> MSVQAEIGILDHVDGSSEF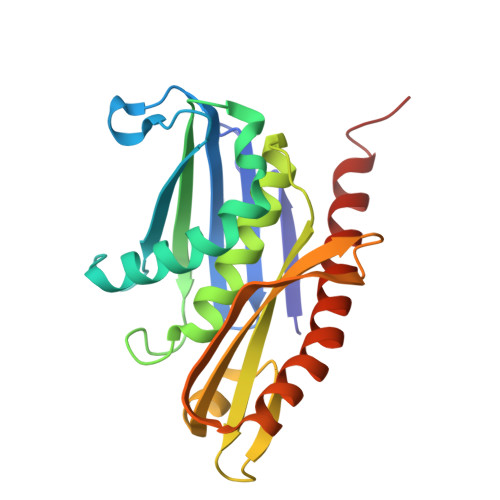VSQDTKVICSVTGPIEPKARQELPTQLALEIIVRPAKGVATTREKVLEDKLRAVLTPLITRHCYPRQLCQITCQILESGEDEAEFSLRELSCCINAAFLALVDAGIALNSMCASIPIAIIKDTSDIIVDPTAEQLKISLSVHTLALEFVNGGKVVKNVLLLDSNGDFNEDQLFSLLELGEQKCQELVTNIRRIIQDNISPRLVV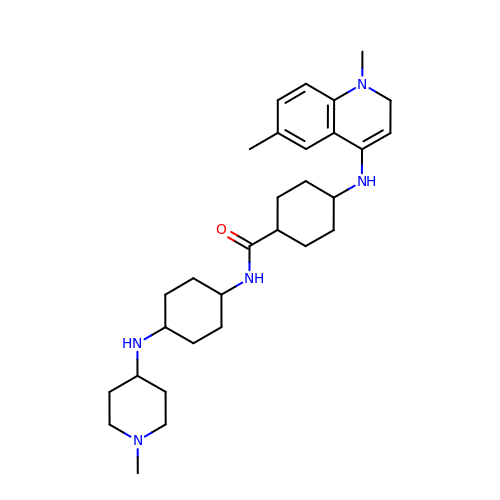1,6-DIMETHYL-4-(4-(4-(1-METHYLPYRIDINIUM-4-YLAMINO)PHENYLCARBAMOYL)PHENYLAMINO)QUINOLINIUM | C30 H47 N5 O | VJDMGOLLSXKCPI-DHBIPOTOSA-N>MVMYFIGLGLYDERDITVKGLEIAKKCDYVFAEFYTSLMAGTTLGR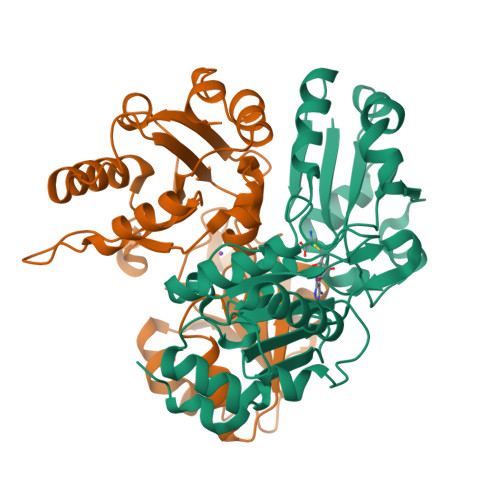IQKLIGKEIRVLSREDVELNFENIVLPLAKENDVAFLTPGDPLVATTHAELRIRAKRAGVESYVIHAPSIYSAVGITGLHIYKFGKSATVAYPEGNWFPTSYYDVIKENAERGLHTLLFLDIKAEKRMYMTANEAMELLLKVEDMKKGGVFTDDTLVVVLARAGSLNPTIRAGYVKDLIREDFGDPPHILIVPGKLHIVEAEYLVEIAGAPREILRVNV[2x]>MKVIDPQHSDKPNVLILGSGWGAISFLKHIDTKKYNVSIISPRSYFLFTPLLPSAPVGTVDEKSIIEPIVNFALKKKGNVTYYEAEATSINPDRNTVTIKSLSAVSQLYQPENHLGLHQAEPAEIKYDYLISAVGAEPNTFGIPGVTDYGHFLKEIPNSLEIRRTFAANLEKANLLPKGDPERRRLLSIVVVGGGPTGVEAAGELQDYVHQDLRKFLPALAEEVQIHLVEALPIVLNMFEKKLSSYAQSHLENTSIKVHLRTAVAKVEEKQLLAKTKHEDGKITEETIPYGTLIWATGNKAR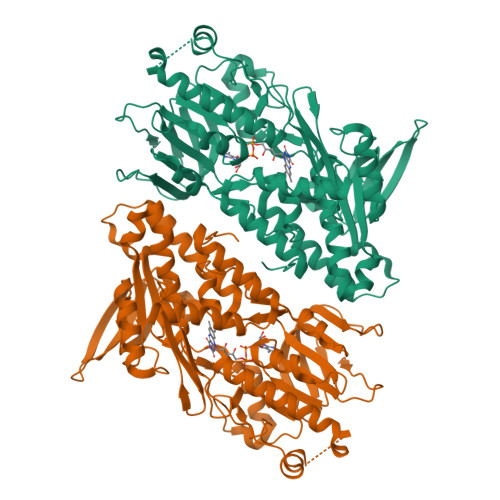PVITDLFKKIPEQNSSKRGLAVNDFLQVKGSNNIFAIGDNAFAGLPPTAQVAHQEAEYLAKNFDKMAQIPNFQKNLSSRKDKIDLLFEENNFKPFKYNDLGALAYLGSERAIATIRSGKRTFYTGGGLMTFYLWRILYLSMILSARSRLKVFFDWIKLAFFKRDFFKGL[2x]>[2x]DLPRHIAVLCDGNRRWARSAGYDDVSY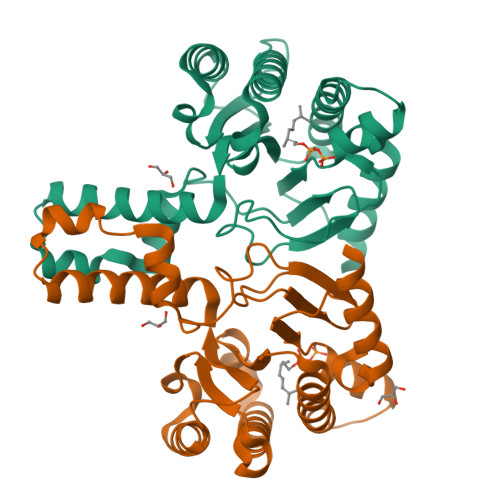GYRMGAAKIAEMLRWCHEAGIELATVYLLSTENLQRDPDELAALIEIITDVVEEICAPANHWSVRTVGDLGLIGEEPARRLRGAVESTPEVASFHVNVAVGYGGRREIVDAVRALLSKELANGATAEELVDAVTVEGISENLYTSGQPDPDLVIRTSGEQRLSGFLLWQSAYSEMWFTEAHWPAFRHVDFLRALRDYSAR>[8x]GPHMGIFPTVEKLVEEMREQLDEVDSHPRTSIFEKLPSK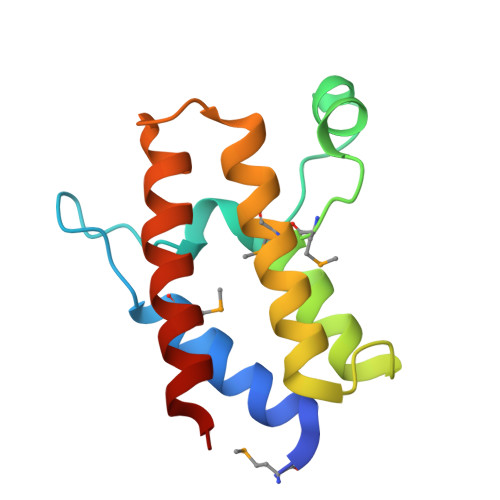RDYPDYFKVIEKPMAIDIILKNCKNGTYKTLEEVRQALQTMFENARFYNEEGSWVYVDADKLNEFTDEWFKEHSS> SMGVRKLATIRTAGEITPIAGAEAIECCHVDGWTCVIKKGEFKQGDRGVYFEIDSFIKEDNDRYPMLSKQVIDYEGQRGTRLRTARLRGQLSQGLFLPMDRFPELASNQVGDDVTEILGITKWEPPISTNLSGEILGEFPTFISKTDQERVQNLIPQIEENKGQKFEVTVKLDGSSMTVYRKDDHIGVCGRNWELRETATNAQWHAARRNKMIEGLQFLNRNLALQGEIIGESIQGNLEKLKGQDFYLFDIYDIDKAQYLTPIERQSLVKQLNDNGFTVKHVPILDDLELNHTAEQILAMADGPSLNKNVKRAGLVFKRLDGKFS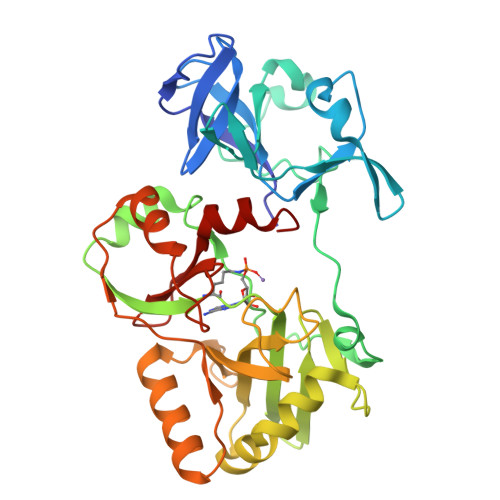FKAISNAYLEKHKDR>MYSKIKISGTIEVVTGLHIGGGGESSMIGAIDSPVVRDLQTKLPIIPGSSIKGKMRNLLAKHFGLKMKQESHNQDDERVLRLFGSSEKGNIQRARLQISDAFFSEKTKEHFAQNDIAYTETKFENTINRLTAVANPRQIERVTRGSEFDFVFIYNVDEESQVEDDFENIEKAIHLLENDYLGGGGTRGNGRIQFKDTNIETVVGEYDSTNLKIK[4x];> MNKKNILMYGSLLHDIGKIIYRSGDHTFSRGTHSKLGHQFLSQFSEFKDNEVLDNVAYHHYKELAKANLDNDNTAYITYIADNIASGIDRRDIIEEGDEEYEKQLFNFDKYTPLYSVFNIVNSEKLKQTNGKFKFSNESNIEYPKTENIQYSSGNYTTLMKDMSHDLEHKLSIKEGTFPSLLQWTESLWQYVPSSTNKNQLIDISLYDHSRITCAIASCIFDYLNENNIHNYKDELFSKYENTKSFYQKEAFLLLSMDMSGIQDFIYNISGSKALKSLRSRSFYLELMLEVIVDQLLERLELARANLLYTGGGHAYLLVSNTDKVKKKITQFNNELKKWFMSEFTTDLSLSMAFEKCSGDDLMNTSGNYRTIWRNVSSKLSDIKAHKYSAEDILKLNHFHSYGDRECKECLRSDIDINDDGLCSICEGIINISNDLRDKSFFVLSETGKLKMPFNKFISVIDYEEAEMLVQNNNQVRIYSKNKPYIGIGISTNLWMCDYDYASQNQDMREKGIGSYVDREEGVKRLGVVRADIDNLGATFISGIPEKYNSISRTATLSRQLSLFFKYELNHLLENYQITAIYSGGDDLFLIGAWDDIIEASIYINDKFKEFTLDKLTLSAGVGMFSGKYPVSKMAFETGRLEEAAKTGEKNQISLWLQEKVYNWDEFKKNILEEKLLVLQQGFSQTDEHGKAFIYKMLALLRNNEAINIARLAYLLARSKMNEDFTSKIFNWAQNDKDKNQLITALEYYIYQIREAD;> MTLATKVFKLSFKTPVHFGKKRLSDGEMTITADTLFSALFIETLQLGKDTDWLLNDLIISDTFPYENELYYLPKPLIKIDSKEEDNHKAFKKLKYVPVHHYNQYLNGELSAEDATDLNDIFNIGYFSLQTKVSLIAQETDSSADSEPYSVGTFTFEPEAGLYFIAKGSEETLDHLNNIMTALQYSGLGGKRNAGYGQFEYEIINNQQLSKLLNQNGKHSILLSTAMAKKEEIESALKEARYILTKRSGFVQSTNYSEMLVKKSDFYSFSSGSVFKNIFNGDIFNVGHNGKHPVYRYAKPLWLEV;>[3x]MTFAHEVVKSNVKNVKDRKGKEKQVLFNGLTTSKLRN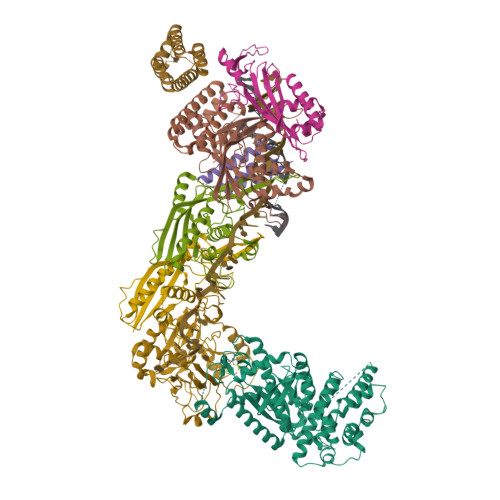LMEQVNRLYTIAFNSNEDQLNEEFIDELEYLKIKFYYEAGREKSVDEFLKKTLMFPIIDRVIKKESKKFFLDYCKYFEALVAYAKYYQKED methyl N-[4-amino-3-(L-arginylamino)benzene-1-carbonyl]-L-tyrosinate 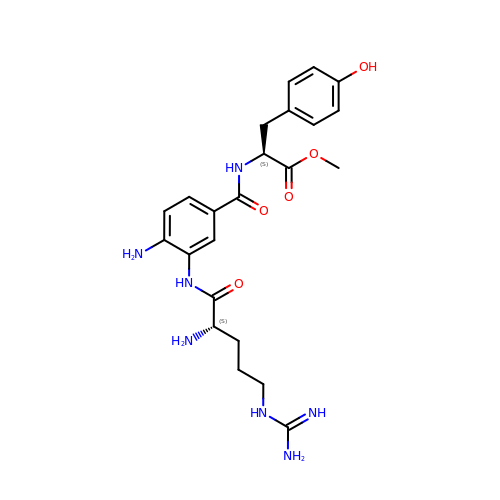| C23 H31 N7 O5 | JECKMXQKZJERLG-HKUYNNGSSA-N> MAAQNEQRPERIKTTPYLEGDVLSSDSGPLLSVFALQEIMQKVRQVQADYMTATREVDFTVPDVQKILDDIKALAAEQVYKIVKVPSISFRHIVMQSRDRVLRVDTYYEEMSQVGDVITEDEPEKFYSTIIKKVRFIRGKGSFILHDIPTRDHRGMEVAEPEVLGVEFKNVLPVLTAEHRAMIQNALDGSIIENGNVATRDVDVFIGACSEPVYRIYNRLQGYIEAVQLQELRNSIGWLERLGHRKRITYSQEVLTDFRRQDTIWVLALQLPVNPQVVWDVPRSSIANLIMNIATCLPTGEYIAPNPRISSITLTQRITTTGPFAILTGSTPTAQQLNDVRKIYLALMFPGQIILDLKIDPGERMDPAVRMVAGVVGHLLFTAGGRFTNLTQNMARQLDIALNDYLLYMYNTRVQVNYGPTGEPLDFQIGRNQYDCNVFRADFATGTGYNGWATIDVEYREPAPYVHAQRYIRYCGIDSRELINPTTYGIGMTYHCYNEMLRMLVAAGKDSEAAYFRSMLPFHMVRFARINQIINEDLHSVFSLPDDMFNALLPDLIAGAHQNADPVVLDVSWISLWFAFNRSFEPTHRNEMLEVAPLIESVYASELSVMKVDMRHLSLMQRRFPDVLIQARPSHFWKAVLNDSPEAVKAVMNLSHSHNFINIRDMMRWVMLPSLQPSLKLALEEEAWAAANDFEDLMLTDQVYMHRDMLPEPR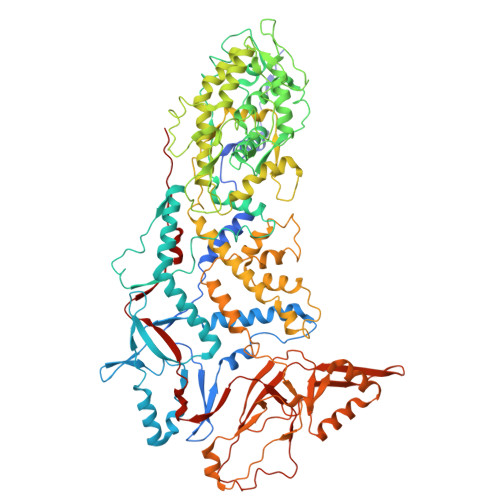LDDIERFRQEGFYYTNMLEAPPEIDRVVQYTYEIARLQANMGQFRAALRRIMDDDDWVRFGGVLRTVRVKFYDARPPDDVLQGLPFSYDTNERGGLAYATIKYATETTIFYLIYNVEFSNTPDSLVLINPTYTMTKVFINKRIVERVRVGQILAVLNRRFVAYKGKMRIMDITQSLKMGTKLAAPTV>MGSSHHHHHHSSGLVPRGSHMASNAYTERDMLQKAADETTLKNVLVMKQAWVPYPAYTDRAAWDSLMGSNKQRLIAAGEKLLDYKWQLIPATAYLEYERTGNRKIMEVPYDANRQALNTLMLAELAEGKGRFIDQLLNGAYMSCEMNSWVLSAHLPRQSSKRSLPDFREQIIDLGSGGYGALMAWVHYFFRKPFDKINPVVSLQMRKAIKERILDPYMNDDDMWWMAFNWQPGEIINNWNPWCNSNALQCFLLMENNKDRLAKAVYRSMKSVDKFINFVKSDGACEEGTSAWGHAAGKLYDYLQILSDGTGGKISLLNEPMIRRMGEYMSRSYVGNGWVVNFADASAQGGGDPLLIYRFGKAVNSNEMMHFAAYLLNGRKPYATMGNDAFRSLQSLLCCNDLAKETPKHDMPDVTWYPETEFCYMKNKNGMFVAAKGGFNNESHNHNDVGTFSLYVNTIPVILDAGVGTYTKQTFGKDRYTIWTMQSNYHNLPMINGIPQKYGQEYKATNTTCNEKKRVFSTDIAAAYPSEAKVKNWIRSYTLDDRKLTITDSYTLEEAVAPNQVNFMTWGNVTFPSQGKIQIEVKGQKVELDYPTLFKAELETIQLDDPRLSNVWGKEIYRITLKTNEKKETGNYKFVIQQIK[2x]

In bacteria, however, a different strategy employing a class of enzyme known as polysaccharide lyases (PL) is deployed. PLs selectively target glycans composed of uronic acids with a C4 hydroxyl group linked to the preceding sugar in the glycan chain. This enables PLs to operate through a β-elimination mechanism that relies on proton abstraction from the C5 carbon of the uronic acid sugar ring, resulting in double bond formation between C4 and C5 and elimination of the preceding sugar. The three characterized PL33_1 enzymes were all from Bacteroides species inhabiting the human colon: BT4410 (BtPL33HA) and BcellWH2_04512 (BcPL33HA) are hyaluronidases from Bacteroides thetaiotaomicron VPI-5482 (B. theta) and Bacteroides cellulosilyticus WH2 (B. cell), respectively, while HMPREF1181_01744 (BsPL33Heparosan) is a heparosanase from Bacteroides stercoris CC31F (B. stercoris). The enzymes are 68% identical and contain a larger N-terminal α-helical (α/α)6 toroid domain (residues 21 to 401; BtPL33HA numbering used throughout this section unless specified) and a smaller β-sheet C-terminal domain (residues 402 to 635).

Based on the Apo structures of BtPL33HA and BcPL33HA, combined with Consurf analysis, a total of 20 BtPL33HA mutants were made in order to understand the roles of individual amino acids in substrate binding and catalysis. This enabled the structural characterization of a catalytically compromised variant (Y291A) of BtPL33HA in complex with a HA tetrasaccharide. The complex contained two molecules of BtPL33HA in the asymmetric unit, with one molecule containing electron density for which a trisaccharide could be modeled, and the other for which a less well-ordered tetrasaccharide could be modeled. The C-terminal domain possesses an extended loop region between β-strands 5 and 6 (Leu455-Leu484: BtPL33HA, and Ile464-Leu493: BcPL33HA), forming an octahedral Zn2+ coordination site [supported by anomalous X-ray diffraction data], along with the loop region between α-helices 12 and 13 from the N-terminal domain. The Zn2+ coordination site is a conserved feature in PL33. A hydrophobic platform composed of W224, W239, L174, and W242 underpins binding at the +2, +1, and −1 subsites, while no obvious interactions occur with the −2 sugar. The +1 subsite, the site of catalysis, is where the majority of interactions occur. The side chain of R103 interacts with the O2 and O3 of the +1 GlcA, while H154 only interacts with O2. N238 interacts with the carboxylate of the +1 GlcA through its amide group, while Y291 lies ~6 Å from C5. To determine whether conformational change accompanies ligand binding, we performed a SAXS experiment with the inactive BtPL33HA Y291A mutant in the presence of a HA tetrasaccharide (this mutant displays residual activity on HA but cannot cleave tetrasaccharides). However, neither the presence of the mutation nor the substrate induced a conformational change as indicated by unaltered scattering profiles.>[2x]MSTFIIRLLIFSLLCGSFSIHAEEQNGMKLERVVIVSRHGVRAPTKFTPIMKNVTPDQWPQWDVPLGWLTPRGGELVSELGQYQRLWFTSKGLLNNQTCPSPGQVAVIADTDQRTRKTGEAFLAGLAPKCQIQVHYQKDEEKNDPLFNPVKMGKCSFNTLQVCNAILERAGGNIELYTQRYQSSFRTLENVLNFSQSETCKTTEKSTKCTLPEALPSELKCTPDNVSLPGAWSLSSTLTEIFLLQEAQGMPQVAWGRITGEKEWRDLLSLHNAQFDLLQRTPEVARSRATPLLDMIDTALLTNGTTENRYGIKLPVSLLFIAGHDTNLANLSGALDLNWSLPGQPDNTPPGGELVFEKWKRTSDNTDWVQVSFVYQTLRDMRDIQPLSLEKPAGKVDLKLIACEEKNSQGMCSLKSFSRLIKEIRVPECAVTE

We here use rational computation-based procedures to design stabilizing disulfide bridges in the phytase from Citrobacter braakii, a biotechnologically important enzyme currently used in RONOZYME HiPhos (DSM Nutritional Products, Basel, Switzerland). At its backbone is a mainly parallel β-sheet, surrounded by α-helices and loops. The second domain, primarily α-helical, is composed of two insertions (residues 39–46 and 136–259) in the first domain and is seen on the left of the Figure in red/yellow.

The structure with a disulfide bridge engineered between residues 141 and 199 was refined to 2.3 Å spacing with two independent protein monomers in the asymmetric unit. The engineered disulfide between residues 141 and 199 crosslinks an α-helix and a coiled loop of the α-helical domain and has well-defined electron density indicating a highly successful introduction of this new element into the phytase fold. The major domain on the right is composed of residues 6–28, 47–135 and 260–410 and is colored blue and grey. The rmsd in ∼380 equivalent Cα positions is 1.18 Å. The four disulfide bridges can be seen to be totally conserved. All the variants showed similar activity levels in the standard phytase assay and essentially identical pH profiles. Furthermore, very similar temperature dependencies of activity are observed at sub-denaturational temperatures while the high temperature activity drop associated with irreversible denaturation is shifted to higher temperatures as the number of disulfide bridges increases. These results suggest that, while the engineered crosslinks do enhance stability, they do not cause dramatic alterations in the native, functional structure of the enzyme, corroborated by the 3D-structure of one of the variants. Indeed, the effects of the engineered disulfides on thermal stability appear to be roughly additive; for instance adding the Tm enhancements (relative to wt) found for the single variants (2.2, 6.3 and 1.3°C for S1, S2 and S3, respectively), ΔTm values of 8.5, 7.6 and 9.8°C are predicted for D1, D2 and T, while the experimental Tm enhancements relative to wt for these variants are 9.8 (D1), 8.2 (D2) and 12.1°C (T).>MAEEIKKILVKEESLRRALHNELQELRGNIRVYCRIRPPLPHEDDNIEHIKVQPFDDDNGDQGMTINRGNSQVIPFKFDKIFDQQETNDEIFKEVGQLIQSSLDGYNVCIFAYGQTGSGKTYTMLNPGDGIVPATINHIFSWIDKLAARGWSYKVSCEFIEIYNENIVDLLRSGAPSQENNDRNADSKHEIRHDQELKTTYITNITTCVLDSRDTVDKVLKRANKLRSTASTAANEHSSRSHSIFIIHLEGKNEGTGEKSQGILNLVDLAGSERLNSSMVVGERLRETQSINKSLSCLGDVIHALNSPDGQKRHIPFRNSKLT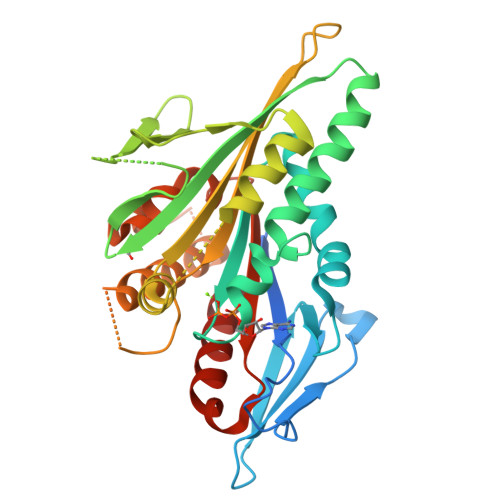YLLQYSLIGSSKTLMFVNISPAALHLNETINSLRFASKVNNTKMITRN[2x]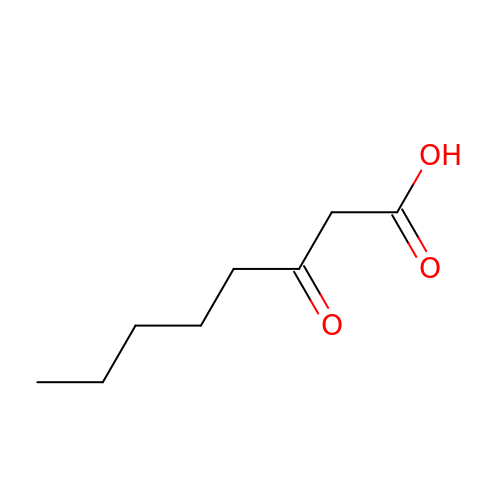3-OXOOCTANOIC ACID | C8 H14 O3 | FWNRRWJFOZIGQZ-UHFFFAOYSA-N>[2x]MIKNEIKILSDIEHIKKRSGMYIGSSANETHERFMFGKWESVQYVPGLVKLIDEIIDNSVDEGIRTKFKFANKINVTIKNNQVTVEDNGRGIPQAMVKTPTGEEIPGPVAAWTIPKAGGNFGDDKERVTGGMNGVGSSLTNIFSVMFVGETGDGQNNIVVRCSNGMENKSWEDIPGKWKGTRVTFIPDFMSFETNELSQVYLDITLDRLQTLAVVYPDIQFTFNGKKVQGNFKKYARQYDEHAIVQEQENCSIAVGRSPDGFRQLTYVNNIHTKNGGHHIDCAMDDICEDLIPQIKRKFKIDVTKARVKECLTIVMFVRDMKNMRLIRQTKERLTSPFGEIRSHIQLDAKKISRDILNNEAILMPIIEAALARKLAAEKAAETKAAKKASKAKVHKHIKANLCGKDADTTLFLTEGDSAIGYLIDVRDKELHGGYPLRGKVLNSWGMSYADMLKNKELFDICAITGLVLGEKAFEEKEDGEWFTFELNGDTIIVNENDEVQINGKWITVGELRKNLMKFVKIDSSSVDMKKYKLQNNVRRSIKSSSMNYANVAIMTDADHDGLGSIYPSLLGFFSNWPELFEQGRIRFVKTPVIIAQVGKKQEWFYTVAEYESAKDALPKHSIRYIKGLGSLEKSEYREMIQNPVYDVVKLPENWKELFEMLMGDNADLRKEWMSQHHHHHH;>[2x]MQLNNRDLKSIIDNEALAYAMYTVENRAIPNMIDGFKPVQRFVIARALDLARGNKDKFHKLASIAGGVADLGYHHGENSAQDAGALMANTWNNNFPLLDGQGNFGSRTVQKAAASRYIFARVSKNFYNVYKDTEYAPVH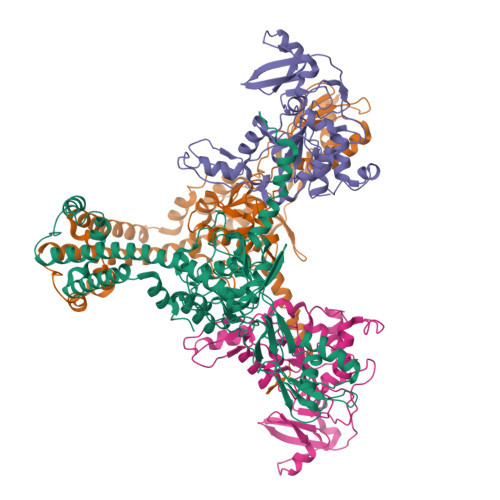QDKEHIPPAFYLPIIPTVLLNGVSGIATGYATYILPHSVSSVKKAVLQALQGKKVTKPKVEFPEFRGEVVEIDGQYEIRGTYKFTSRTQMHITEIPYKYDRETYVSKILDPLENKGFITWDDACGEHGFGFKVKFRKEYSLSDNEEERHAKIMKDFGLIERRSQNITVINEKGKLQVYDNVVDLIKDFVEVRKTYVQKRIDNKIKETESAFRLAFAKAHFIKKVISGEIVVQGKTRKELTEELSKIDMYSSYVDKLVGMNIFHMTSDEAKKLAEEAKAKKEENEYWKTTDVVTEYTKDLEEIKHHHHHHHHHH3-(PHOSPHONOMETHYL)PYRIDINE-2-CARBOXYLIC 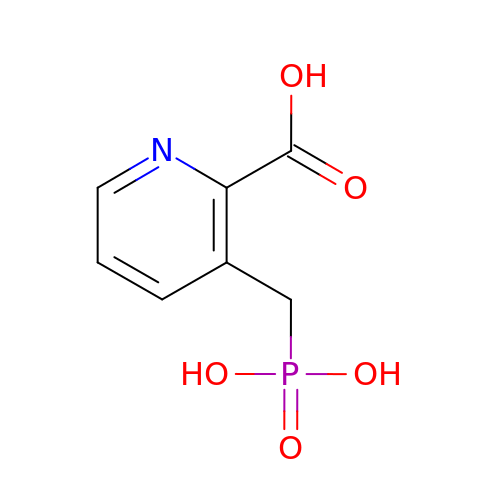ACID | C7 H8 N O5 P | ROSWJUKEABEPFJ-UHFFFAOYSA-N> GAGCAGACCTGA;> CGGCACTCA;> TCACCG;> TCTGAGTGGGTCTGC

In this work, we exhaustively probe the ability of all 36 immobile HJ sequences to form DNA crystals in two different designed systems. Three separate self-assembling DNA crystal systems are described in this report: the “4 × 5” and “4 × 6” designs (collectively referred to as the 4 × N systems), and a third construct with a “scrambled” sequence variant of the 4 × 6 lattices. Self-assembly was mediated by three constituent oligonucleotides: (S1) containing four sequence repeats of either 5 or 6 bases; (S2) composed of 21 bases containing complementary regions to both (S1); and (S3) which forms the second junction crossover. The HJ serves as the fundamental component at the core of each unit, and the ultimate assembly of the full lattice is facilitated by the complementary 2-base sticky ends that tail each duplex.

Each asymmetric unit could be defined as either a HJ containing 10 and 11 bp on each arm, or as a 21-bp linear duplex. In parallel, we employed the previously reported J1 4 × 6 system (3.05 Å), with P32 symmetry. Seventeen of the 36 junctions successfully crystallized, a 47% success rate. Although in the majority of cases, the individual junctions, regardless of design parameters, had a preference for crystallizing in cacodylic acid within the 6.0–6.5 pH regime, not all crystals were confined to this requirement. In the 4 × 5 system, J25 and J34, both displaying P32 symmetry, crystallized in 50 mM Tris pH = 8.0 buffer containing cobalt hexamine (CoH18N6) and 10 mM MgCl2, and 50 mM HEPES pH = 7.5 with 20 mM MgCl2, respectively. Only cobalt could account for the different peaks in the Fo–Fc maps in J25, whereas in J34, and J22 and J23 in the 4 × 6 and 4 × 6 scramble systems, respectively, contained Mg2+. The modeled ions were readily superimposable, and well-coordinated at Pos1 & 2.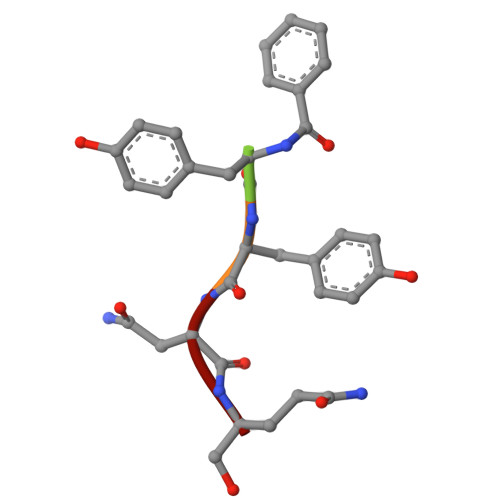> XYYNQ> MEPAMEPETLEARINRATNPLNKELDWASINGFCEQLNEDFEGP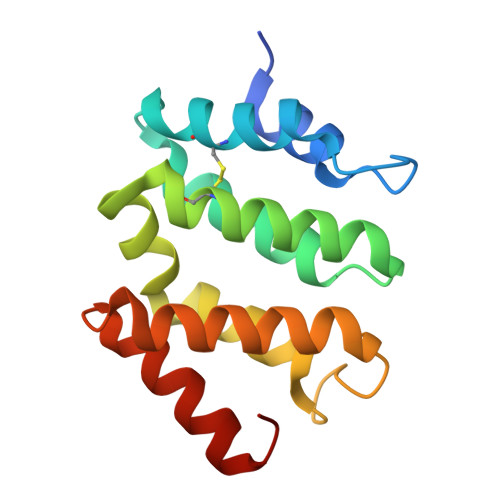PLATRLLAHKIQSPQEWEAIQALTVLETCMKSCGKRFHDEVGKFRFLNELIKVVSPKYLGSRTSEKVKNKILELLYSWTVGLPEEVKIAEAYQMLKKQGIVKS>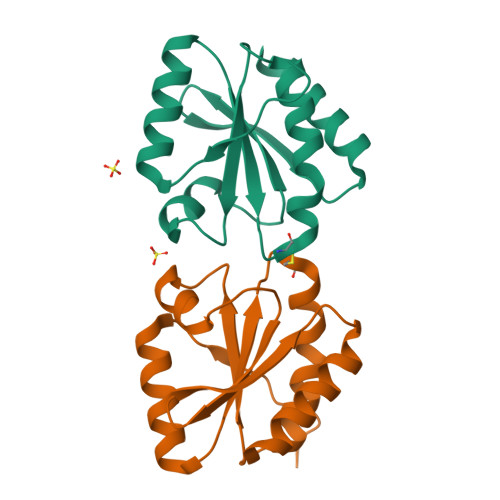[2x]MATRPTSVEMEPIDDSHHLDKILLQARELSQPIIIDWMASWCRKSIYLKPKLEKLAAEYDTKIKFYSADVNKVPQALVKRGNISKMPTIQLWKDGEMKAEVIGGHKAWLVIEEVREMIQKFV> GPMADLWDDNDDDDDILELVNRPPMSQMAVPIKPPESQAEQLMKAKGEVGVLRQ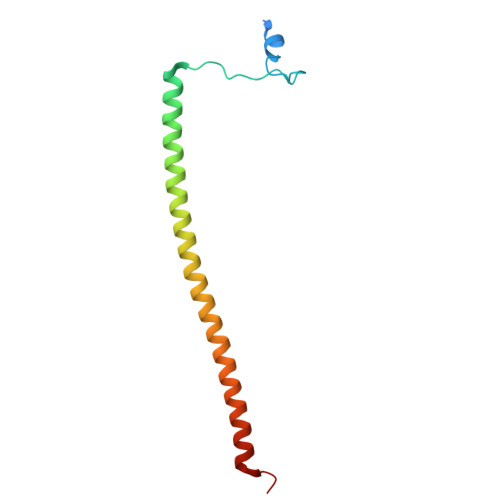KLSMLEKTLREHDDNQKKLESSLKSSHEEEVTKLKIELERLEDERKFMLLEQKHLFT> PMARTRYGPVIGKVEQGALAFKGIPYGAPTSGSGRFMPPTPPQPWSTPLRAFDYGPTAPQSDPQDALESGAADARESEDCLTLNVWTPSLNDQRKRPVMVWLHGGGLWRLSAAGDYQAGTHLAAHSDVVMVSPNHRLNVLAHAYLDEYDPAFAGSSSAGMLDLVLALKWVRDNIEEFGGDPDNVTIFGQSGGGQKVSFLMAMPAAAGLFHKAIIQSGPAPLALEKPYARELSARLLTLLDIPKNRVRDIQNVPLDAIMRAYYQI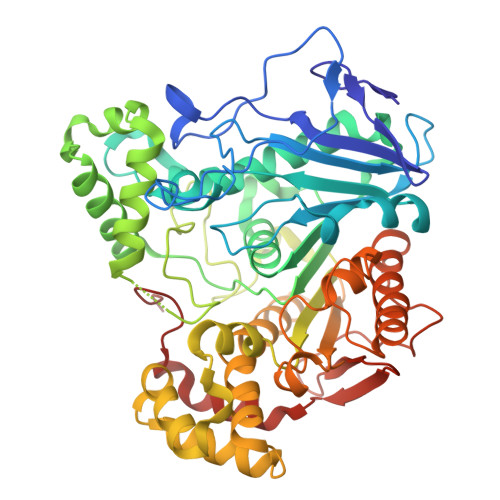FEELGGFGVMGVIQDFAPVVDDVALPQHPFWNGASPLSRDVPLMIGCTRTEMTEYFLASNPGAAKRDFAAVTAQLEPVFGMQAPAVVAHYRATHPTASPWEVDALIRSDWPTRLFTQRIADEQVKLGGAPVWMYRMDWQTTARDGLLMSPHAIDIPFVLDTVGTEPVEPGQLAEQQRMMQQMNNAWVSFARNGNPQNKYIPPWQPYNSTSRPTMIFNLHSHMANDPDGSDLAFLKKDLANLEVVAGGVTH>[2x]VIEKVQHIQLLQKNVRAQLVDMKRLEVDIDIKIRSCRGSCSRALAREVDLKDYEDQQKQLEQVIAK;>HQL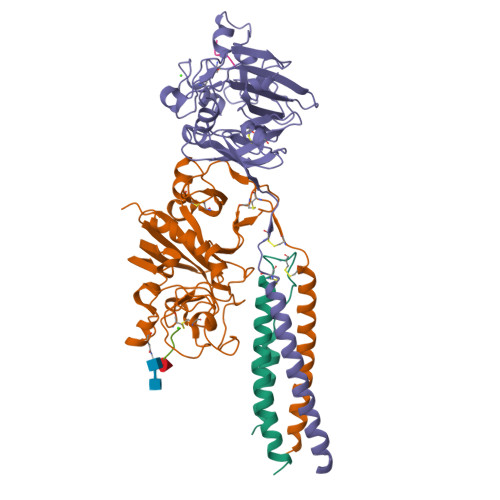YIDETVNSNIPTNLRVLRSILENLRSKIQKLESDVSAQMEYCRTPCTVSCNIPVVSGKECEEIIRKGGETSEMYLIQPDSSVKPYRVYCDMNTENGGWTVIQNRQDGSVDFGRKWDPYKQGFGNVATNTDGKNYCGLPGEYWLGNDKISQLTRMGPTELLIEMEDWKGDKVKAHYGGFTVQNEANKYQISVNKYRGTAGNALMDGASQLMGENRTMTIHNGMFFSTYDRDNDGWLTSDPRKQCSKEDGGGWWYNRCHAANPNGRYYWGGQYTWDMAKHGTDDGVVWMNWKGSWYSMRKMSMKIRPFFPQQ[2x];>YEASILTHDSSIRYLQEIYNSNNQKIVNLKEKVAQLAAQCQEPCKDTVQIHDITGKDCQDIANKGAKQSGLYFIKPLKANQQFLVYCEIDGSGNGWTVFQKRLDGSVDFKKNWIQYKEGFGHLSPTGTTEFWLGNEKIHLISTQSAIPYALRVELEDWNGRTSTADYAMFKVGPEADKYRLTYAYFAGGDAGDAFDGFDFGDDPSDKFFTSHNGMQFSTWDNDNDKFEGNCAEQDGSGWWMNKCHAGHLNGVYYQGGTYSKASTPNGYDNGIIWATWKTRWYSMKKTTMKIIPFNRLTIGEGQQHHLGGAK[2x];>[4x]GHRP~{N}-[[(2~{R},3~{S},4~{R},5~{R})-5-[8-[3-[[(2~{R},3~{S},4~{R},5~{R})-5-(6-aminopurin-9-yl)-3,4-bis(oxidanyl)oxolan-2-yl]methoxy]prop-1-ynyl]-6-azanyl-purin-9-yl]-3,4-bis(oxidanyl)oxolan-2-yl]methyl]-4-azanyl-butanamide 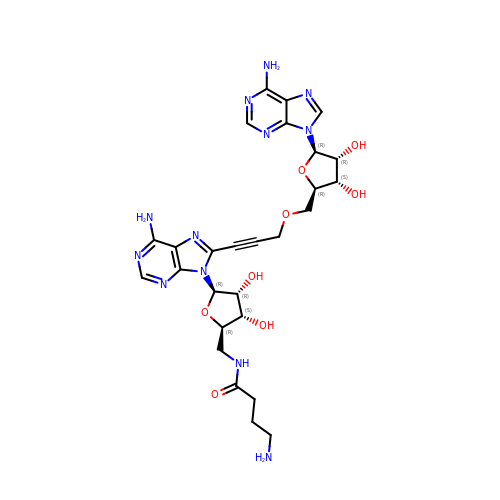| C27 H34 N12 O8 | FSTDOBBDPHECFF-GMIOVBLFSA-N>GPMESNNGIILRVAEANSTDPGMSRVRLDESSRRLLDAE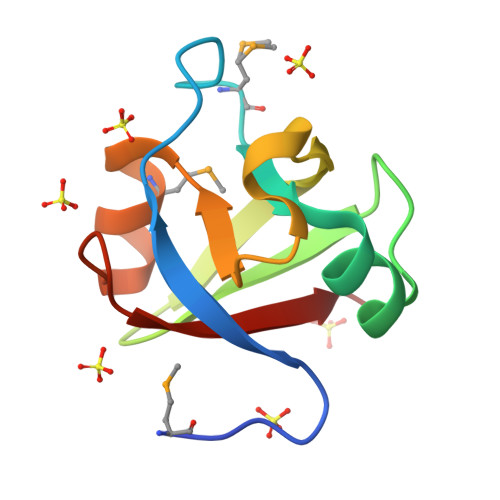IGDVVEIEKVRKTVGRVYRARPEDENKGIVRIDSVMRNNCGASIGDKVKVRKVR[2x]> MYQRTRFLWSSWRDYPLGSRDRRGRFNMDEAAAALQLNPAYAAALYRPLNYTFHIRGQLYPAQKGRPSRPGSLAASQGRMFPLYQRNDRLDKELFRL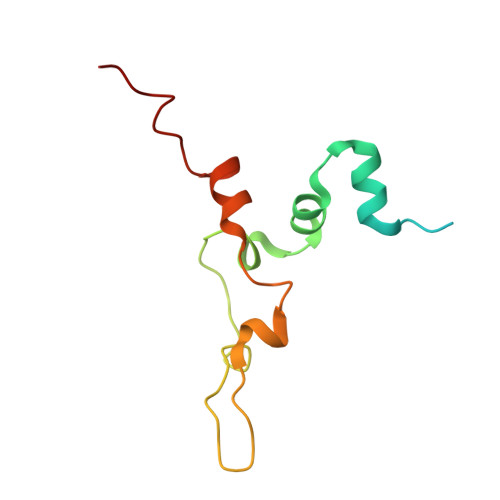NSRGLTTE The mycobacterial membrane protein large 3 (MmpL3) transporter is essential and required for shuttling the lipid trehalose monomycolate (TMM), a precursor of mycolic acid (MA)-containing trehalose dimycolate (TDM) and mycolyl arabinogalactan peptidoglycan (mAGP), in Mycobacterium species, including Mycobacterium tuberculosis and Mycobacterium smegmatis. A detailed analysis suggested that MmpL3 is a TMM flippase that is absolutely essential for transporting TMMs across the cell membrane. MmpL3 consists of 12 transmembrane helices (TMs 1 to 12) and 2 periplasmic subdomains (PDs 1 and 2). Our structural data are in line with MD simulations that indicate the major conformational change of the transporter is located at the periplasmic subdomain PD2, where this movement can easily be interpreted as a rigid body rotational motion of PD2 in relation to the PD1 subdomain.

To answer this question, we delipidated and purified MmpL3 in a solution containing 0.01% glycol-diosgenin (GDN) detergent. We then determined the cryo-EM structure of MmpL3 surrounded by GDN detergent micelles at a nominal resolution of 2.94 Å (MmpL3-GDN). The density modification program allowed us to improve the resolution of the cryo-EM map to 2.40 Å. The structures of MmpL3-GDN and MmpL3-ND largely resemble each other. However, there are conformational differences between the two. Superimposition of these 2 structures gives rise to an RMSD of 1.4 Å (for 710 Cα atoms), suggesting that these conformations are distinct from each other. The calculated volume of the periplasmic central cavity of GDN solubilized MmpL3 using CASTp 3.0 is 1,716 Å3, which is similar, albeit smaller, to that of the protein embedded in nanodiscs. A detailed inspection on these 2 structures suggests that there is a relative rotational motion involved between the periplasmic subdomains PD1 and PD2 of the MmpL3 membrane protein, where PD2 is found to rotate by 6° in relation to PD1 of MmpL3-GDN when compared with the structure of MmpL3-ND. However, the structures of MmpL3-GDN and MmpL3-TMM II represent the fully open channel conformations.

> MFAWWGRTVYQFRYIVIGVMVALCLGGGVYGISLGNHVTQSGFYDEGSQSVAASLIGDEVYGRDRTSHVVAILTPPDDKKVTDKAWQKKVTEELDQVVKDHEDQIVGWVGWLKAPDTTDPTVSAMKTQDLRHTFISIPLQGDDDDEILKNYQVVEPELQQVNGGDIRLAGLNPLASELTGTIGEDQKRAEVAAIPLVAVVLFFVFGTVIAAALPAIIGGLAIAGALGIMRLVAEFTPVHFFAQPVVTLIGLGIAIDYGLFIVSRFREEIAEGYDTEAAVRRTVMTSGRTVVFSAVIIVASSVPLLLFPQGFLKSITYAIIASVMLAAILSITVLAAALAILGPRVDALGVTTLLKIPFLANWQFSRRIIDWFAEKTQKTKTREEVERGFWGRLVNVVMKRPIAFAAPILVVMVLLIIPLGQLSLGGISEKYLPPDNAVRQSQEQFDKLFPGFRTEPLTLVMKREDGEPITDAQIADMRAKALTVSGFTDPDNDPEKMWKERPANDSGSKDPSVRVIQNGLENRNDAAKKIDELRALQPPHGIEVFVGGTPALEQDSIHSLFDKLPLMALILIVTTTVLMFLAFGSVVLPIKAALMSALTLGSTMGILTWMFVDGHGSGLMNYTPQPLMAPMIGLIIAVIWGLSTDYEVFLVSRMVEARERGMSTAEAIRIGTATTGRLITGAALILAVVAGAFVFSDLVMMKYLAFGLLIALLLDATIIRMFLVPAVMKLLGDDCWWAPRWMKRVQEKLGLGETELPDERKRPTVRESETDQRALVGVGAPPPPPRPHDPTHPAPEPVRPMPPMRSNAPSAAGTARISTPPQPPQPPQAPAQQAGDEPATTRFAMARNAVRNAVNSAVHGGAGSAAAPTERAPRPGGPAQPPAPPQREEREIESWLGALRGPAPAKNVPQPPAQPQRPSTDTTRAMPPQGRPPAGPADRGNENAPTTAFSAQRPPNGGAPADATTAIPTPPQREQEPSTEKLNTREDAPEDPETKRRGGGMSAQDLLRREGRL Here we use a robust deep learning pipeline to design complex folds and soluble analogues of integral membrane proteins. Unique membrane topologies, such as those from G-protein-coupled receptors, are not found in the soluble proteome, and we demonstrate that their structural features can be recapitulated in solution. Biophysical analyses demonstrate the high thermal stability of the designs, and experimental structures show remarkable design accuracy. The soluble analogues were functionalized with native structural motifs, as a proof of concept for bringing membrane protein functions to the soluble proteome, potentially enabling new approaches in drug discovery.

We started by designing soluble analogues of the claudin fold, a class of proteins involved in the formation of tight junctions, which are critical in controlling the flow of molecules between layers of epithelial and endothelial cells. Claudin folds are composed of an α/β mixed secondary structure in which there are four transmembrane α-helices and an extracellular β-sheet. We tested 13 designs for the claudin-like fold (CLF), of which ten were found to be expressed in soluble form. Five designs were further biochemically characterized; three were monomers in solution according to size-exclusion chromatography with multi-angle light scattering (SEC–MALS) and were folded, with two showing a melting temperature (Tm) above 90 °C. The CLF designs showed sequence identity below 13% relative to the native fold and nearest e-values to natural sequences below 0.063. The CLF design series showed that our approach could be used successfully to design soluble analogues of membrane proteins with simple membrane-spanning topologies such as four-helix bundles. To assess the design accuracy, we attempted to crystallize the soluble analogues of membrane topologies and obtained high-resolution X-ray structures for one claudin, one rhomboid protease and two GPCR designed folds. The CLF_4 structure exhibited exceptional design precision in both backbone and side chains, as indicated by an r.m.s.d.Cα of 0.73 Å and r.m.s.d.fa of 1.28 Å. Comparison between CLF_4 and the native claudin demonstrated accurate secondary structural element positioning, with an r.m.s.d.Cα of 3.63 Å and most of the deviation arising from the β-sheet region. In addition, the four helices were mostly hydrophilic, as evidenced by the low lipophilicity potential on the surface.

>[2x]MNEEKREELLEEAKRLLEESLKLLKQAYNTPIEIDLPISGGVKAILYNGKVYLIYENGKVEEIEIPEDDILYPIYNKYIETLKEALKTVEKLQEELEELLENEEDGELSEEERLEKLKELAEELKETAEKLLKSIEEFSKFLEELKKKLPKNIKLNINYSSINLAKEAAEKALEASELLEEVYESSGSGHHHHHH> MGPYLQILEQPKQRGFRFRYVCEGPSHGGLPGASSEKNKKSYPQVKICNYVGPAKVIVQLVTNGKNIHLHAHSLVGKHCEDGVCTVTAGPKDMVVGFANLGILHVTKKKVFETLEARMTEACIRGYNPGLLVHSDLAYLQAEGGGDRQLTDREKEIIRQAAVQQTKEMDLSVVRLMFTAFLPDSTGSFTRRLEPVVSDAIYDSKAPNASNLKIVRMDRTAGCVTGGEEIYLLCDKVQKDDIQIRFYEEEENGGVWEGFGDFSPTDVHRQFAIVFKTPKYKDVNITKPASVFVQLRRKSDLETSEP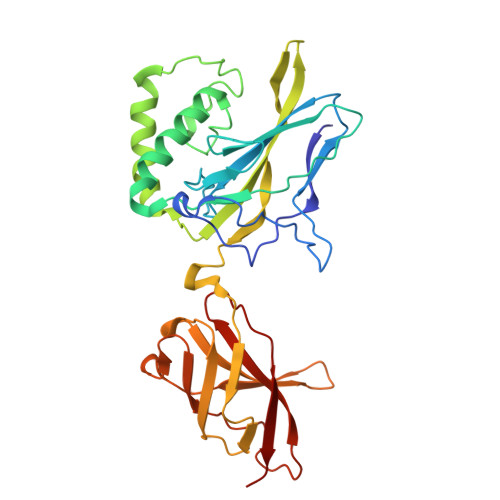KPFLYYPE5-(2-ethylphenyl)thiophene-2-carboxylic acid | C13 H12 O2 S | 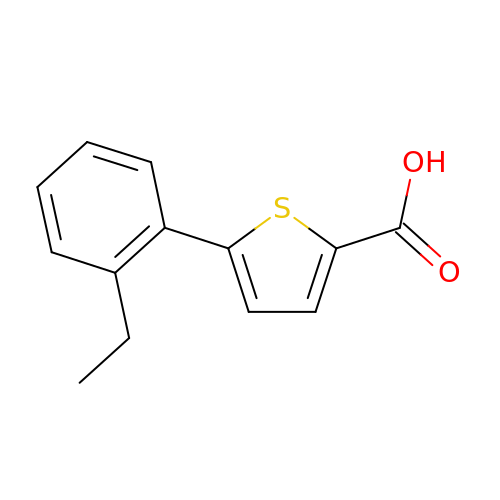MVIOXXJJRFAADN-UHFFFAOYSA-N> MCGRIAQKSAPEDYVEILWPNARLIFDDVAGPRYNIPPGTRPLTMHRLVDQAEALARLPWGYKPHGSSFFMINAKLETIERH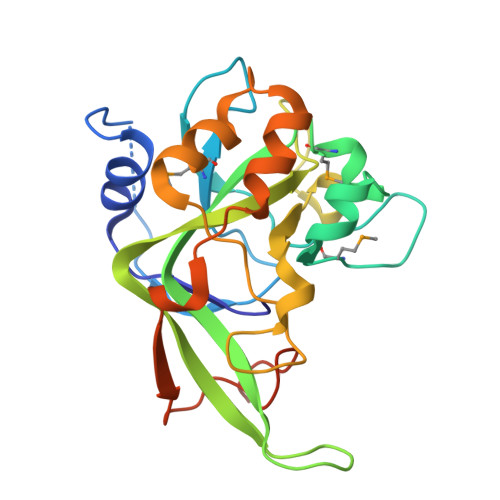GWPWKLMIGTGRILVPADGWYEWKALDSGPKPAKQPYYIHGDAPLLFAGLSAWRRGAELDEAHGFAIVTNDALGGMVDVHDRRPVALPPELAREWVDPATPVARAKEILRAGLPETAFSWYPVRQEVGSSKYQLPDAVDPLLEHHHHHH> ETGKADRYKSHGKGYNWGNYNTETQKCEIFNVKPTCLINNAAYIATTALSHPIEVEGGGGSGGGGSGGGGSGGGGSNYMGNPWTEYMAKYDIEEVHGSGIRVDLGEDAEVAGTQYRLPSGKCPVFGKGIIIENSNTAFLTPVATGNQYLKDGGFAFPPTEPLMSPMTLDEMRHFYKDNKYVKNLDELTLCSRHAGNMIPDNDKNSNYKYPAVYDDKDKKCHILYIAAQENNGPRYCNKDESKRNSMFCFRPAKDISFQNYAYLSKNVVDNWEKVCPRKNLQNAKFGLWVDGNCEDIPHVNEFPAIDLFECNKLVFELSASDQPKQYEQHLTTQQAKDIGAGPVASCFTTRMSPPQQICLNSVVNTALSGTKHHHHHH

The malaria merozoite protein apical membrane antigen 1 (AMA1) is critical for RBC invasion and is one of the most promising blood-stage vaccine candidates. AMA1 binds to RON2 through a surface exposed loop (RON2L) to anchor the parasite to the host cell membrane prior to internalization into a parasitophorous vacuole. Here, three single-component AMA1-RON2L immunogens were designed that retain the structure of the two-component AMA1-RON2L complex: one structure-based design (SBD1) and two insertion fusions. We determined the X-ray crystal structures of SBD1 and insertion fusion immunogens 2 and 3 to resolutions of 1.80 Å, 1.85 Å, and 2.10 Å, respectively.

We used structure-based design (SBD) to alter the location of the C-terminus, enabling seamless attachment of RON2L. The SBD1 immunogen is a circular permutation of AMA1 that contains a Gly/Ser linker (GGGGS × 4) between the original N- and C- termini. The DII loop (358-TDYEKIKEGFKNKNASMIKSAFLPTGAF-385) is removed in SBD1 to produce novel N- and C-termini at residues Lys386 and Thr357, respectively. This new AMA1 C-terminus is immediately adjacent to the N-terminal helix of bound RON2L. Some of the residues deleted in SBD1 (360-YEKIKEGFK-368) comprise a helix in AMA1, which is replaced by the N-terminal helix of RON2L (4-QQAKDIGAG-12). This design approach ensures that the RON2L sequence (3-TQQAKDIGAGPVASCFTTRMSPPQQICLNSVVNTALS-39) could be appended without a linker to create SBD1. The SBD1 structure was most similar to the AMA1-RON2L complex, with no major structural reorganization observed and a Cα root mean square deviation (RMSD) of 0.299 over 245 C-alpha residues. All groups had potent GIA against Plasmodium falciparum 3D7, and there were insignificant differences in IC50 among the AMA1 DI-DII, AMA1 DI-DII-RON2L complex and SBD1 immunogen groups. Strikingly, when the same pooled IgGs were tested with Plasmodium falciparum FVO and Plasmodium falciparum Dd2, only pooled IgGs from the AMA1 DI-DII-RON2L complex and SBD1 immunogen groups showed >50% inhibition at 5 mg/mL, and the IC50 for the SBD1 immunogen group was significantly lower (i.e., more potent) than that for the AMA1 DI-DII-RON2L complex group in both strains (P < 0.001). In conclusion, the single-component SBD1 immunogen elicited potent strain-transcending growth inhibition that was significantly better than that elicited by AMA1 DI-DII alone or the AMA1 DI-DII-RON2L complex despite lacking receptor blocking antibodies that prevent RON2L binding to AMA1.> GSVGPKTGEENQVLVPNLNPTPENLEVVGDGFKITSSINLVGEEEADENAVNALREFLTANNIEINSENDPNSTTLIIGEVDDDIPELDEALNGTTAENLKEEGYALVSNDGKIAIEGKDGDGTFYGVQTFKQLVKESNIPEVNITDYPTVSARGIVEGFYGTPWTHQDRLDQIKFYGENKLNTYIYAPKDDPYHREKWREPYPESEMQRMQELINASAENKVDFVFGISPGIDIRFDGDAGEEDFNHLITKAESLYDMGVRSFAIYWDNIQDKSAAKHAQVLNRFNEEFVKAKGDVKPLITVPTEYDTGAMVSNGQPRAYTRIFAETVDPSIEVMWTGPGVVTNEIPLSDAQLISGIYDRNMAVWWNYPVTDYFKGKLALGPMHGLDKGLNQYVDFFTVNPMEHAELSKISIHTAADYSWNMDNYDYDKAWNRAIDMLYGDLAEDMKVFANHSTRMDNKTWAKSGRE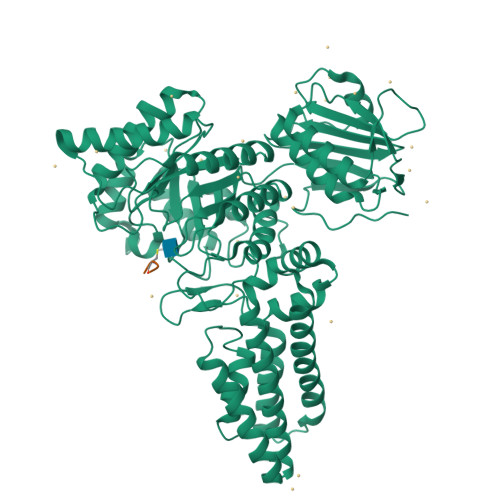DAPELRAKMDELWNKLSSKEDASALIEELYGEFARMEEACNNLKANLPEVALEECSRQLDELITLAQGDKASLDMIVAQLNEDTEAYESAKEIAQNKLNTALSSFAVISEKVAQSFIQEALSFA> GLFDKLKSLVSDDKKDTGTIEIIAPLSGEIVNIEDVPDVVFAEKIVGDGIAIKPTGNKMVAPVDGTIGKIFETNHAFSIESDSGVELFVHFGIDTVELKGEGFKRIAEEGQRVKVGDTVIEFDLPLLEEKAKSTLTPVVISNMDEIKELIKLSGSVTVGETPVIRIKK;> TEKKYIVALDQGTTSSRAVVMDHDANIISVSQREFEQIYPKPGWVEHDPMEIWATQSSTLVEVLAKADISSDQIAAIGITNQRETTIVWEKETGKPIYNAIVWQCRRTA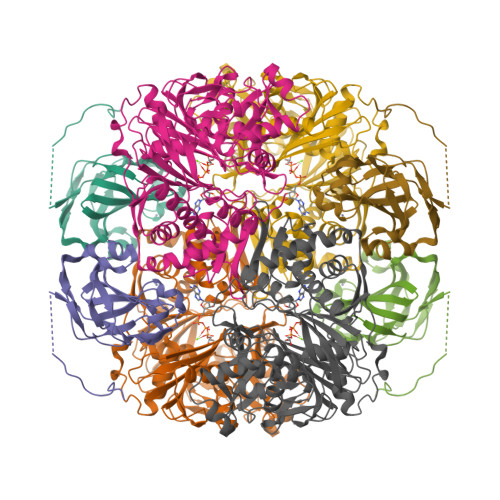EICEHLKRDGLEDYIRSNTGLVIDPYFSGTKVKWILDHVEGSRERARRGELLFGTVDTWLIWKMTQGRVHVTDYTNASRTMLFNIHTLDWDDKMLEVLDIPREMLPEVRRSSEVYGQTNIGGKGGTRIPISGIAGDQQAALFGQLCVKEGMAKNTYGTGCFMLMNTGEKAVKSENGLLTTIACGPTGEVNYALEGAVFMAGASIQWLRDEMKLINDAYDSEYFATKVQNTNGVYVVPAFTGLGAPYWDPYARGAIFGLTRGVNANHIIRATLESIAYQTRDVLEAMQADSGIRLHALRVDGGAVANNFLMQFQSDILGTRVERPEVREVTALGAAYLAGLAVGFWQNLDELQEKAVIEREFRPGIETTERNYRYAGWKKAVKRAMAWEEHDE> GSHMMGNKQTVFTHEQLEAYQDCTFFTRKEIM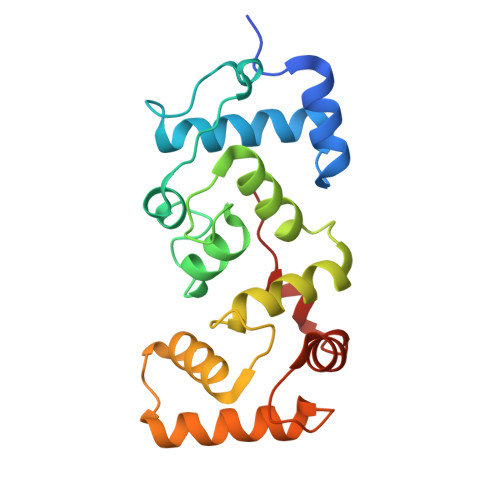RLFYRYQDLAPQLVPLDYTTCPDVKVPYELIGSMPELKDNPFRQRIAQVFSEDGDGHMTLDNFLDMFSVMSEMAPRDLKAYYAFKIYDFNNDDYICAWDLEQTVTKLTRGELSAEEVSLVCEKVLDEADGDHDGRLSLEDFQNMILRAPDFLSTFHIRI HUH endonucleases are diverse enzymes that contain an eponymous motif consisting of a pair of conserved metal-coordinating histidine (H) separated by a bulky hydrophobic residue (U). Replication-initiating HUH endonucleases (Reps) are sequence-specific nucleases that cleave and rejoin single-stranded DNA (ssDNA) during rolling-circle replication. Replication initiator proteins (Reps) from this HUH endonuclease superfamily are found in a variety of bacterial plasmids and viral genomes, including circular Rep-encoding single-stranded DNA (CRESS-DNA) viruses that are known to infect organisms across all three domains of life (1–5). These enzymes initiate rolling-circle replication through sequence-specific processing of the viral single-stranded DNA (ssDNA) genome via cleavage and subsequent phosphotyrosine covalent linkage to the ssDNA’s newly exposed 5′ end. Following linkage, the genome’s freed 3′-OH can be used as a primer for DNA replication before its ultimate return to the active site, where it attacks the phosphotyrosine intermediate to rejoin and release the circular ssDNA genome.

To better understand the roles that coordinated divalent ions play in Rep function, we resolved two cocrystal structures of the endonuclease domain of DCV Rep in complex with a cognate ssDNA 10-mer (5′-TATTATTACC-3′) derived from the DCV Ori, with and without manganese coordinated in the active site. Precleavage complexes were obtained using the dDCV mutant. The substrate in both structures conforms to the characteristic “U”-shaped architecture, indicating that the ssDNA conformation is largely facilitated by the DNA binding interface and intramolecular base pairing and base stacking, with little support from the coordinated cation. Interestingly, four waters occupy the active site in the absence of Mn2+ coordination, and the ion-coordinating triad side chains shift slightly away from the direction of the space occupied by the cation in the Mn2+-bound structure. Indeed, Lys94 is positioned away from the active site in the absence of Mn2+ coordination. However, we observed a notable loss of 19 total contacts (4 of which are hydrogen bonds) at position T−1 when Mn2+ is not present, indicating a dynamic localized conformational shift in that region. In the absence of Mn2+, the measured distance is 3.0 Å, whereas when Mn2+ is coordinated in the active site, and the scissile phosphate is pulled 0.7 Å closer to the oxygen, with a measured distance of 2.3 Å. The bound ssDNA retains its stabilizing intramolecular WC base pair and base stacking regardless of ion coordination. This suggests that while the ion does play an important role in both substrate polarization and positioning, it has little impact on its conformation, which is largely enforced by the nucleic acid’s intramolecular interactions and contacts with the Rep’s sDBM.

>MAKSGNYSYKRWVFTINNPTFEDYVHVLEFCTLDNCKFAIVGEEKGANGTPHLQGFLNLRSNARAAALEESLGGRAWLSRARGSDEDNEEFCAKESTYLRVGEPVSKGRSS[2x]2-[(1-methyl-4-oxidanyl-7-phenoxy-isoquinolin-3-yl)carbonylamino]ethanoic 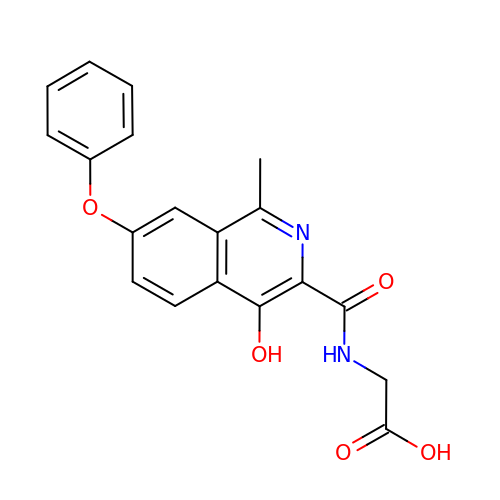acid | C19 H16 N2 O5 | YOZBGTLTNGAVFU-UHFFFAOYSA-N To make further progress, we present here a first characterization of a novel tetrameric ion channel, referred to as NaKTs, with an unusual proline-rich selectivity filter sequence using X-ray crystallography, electrophysiology and MD simulations. Single-channel recordings demonstrate that the NaKTs channel is a Ca2+-activated non-selective cation channel. The NaKTs channel belongs to the family of channels with fourfold symmetric tetrameric pore domains. The X-ray structures revealed the presence of Ca2+ binding sites, SCa, formed by main chain atoms of residues Pro63, Gly65, Ser59 and Leu62, near the intracellular end of the selectivity filter.

The crystallographic structure determined at 3.15 Å displays Ca2+ ions bound to the channel tetramer within the selectivity filter. The structural model is complete over all regions, except for residues 1–3 at the N-terminal and residues 107–123 at the C-terminal regions (the latter might have been cleaved by chymotrypsin digestion). In its broad features, the structure of the NaKTs channel is similar to that of other tetrameric pore domains, with a TM helical segment-labelled M1 (residues 21–45), a pore helix (residues 49–62), the selectivity filter (residues Pro63-Met64-Gly65-Asn66-Gly67-Pro68) and a M2 helix (residues 73–101). The channel is in a conformation with an open intracellular gate, with a strong bend of ∼50° near the centre of the M2 helix. While the open conformation of NaKTs is similar to that observed in previous X-ray structures of other channels, the strongest bend in the M2 helix occurs at the level of residue Val87 rather than at the level of a glycine residue proposed to act as a conserved gating hinge in several channels. The narrowest point along the intracellular vestibule occurs at the level of residue Val92, its side chain pointing towards the central channel axis. The diameter is on the order of 10 Å, which is slightly smaller than that observed in other channels in an open conformation, for example, NaK (10.3 Å at Phe92) and MthK (12.9 Å at Ala88). Three different diffraction datasets were analyzed to identify different ion occupancy states (by virtue of the I4 space group symmetry, the six monomers yield three crystallographically related tetramers). A total of nine crystallographically distinct tetramers were considered in the analysis, revealing four different occupancy states, I to IV, with 0, 2, 3 and 6 Ca2+ ions, respectively.

>MLGLTLMFKRFFGAVRTSWRDPSTRGAVLSLAIIVTAATIFYTLAEKWSVIDSLFYAVSVGLPMGNGPLSPTLTLSKIFTLVYAILVVGLFVTVGGSLASAIVQNNTEKFKRLNRKGSAEAEDHHHHHH[6x]[(1R,5S)-8-AZABICYCLO[3.2.1]OCTAN-3-YL] BENZOATE | C14 H17 N O2 | 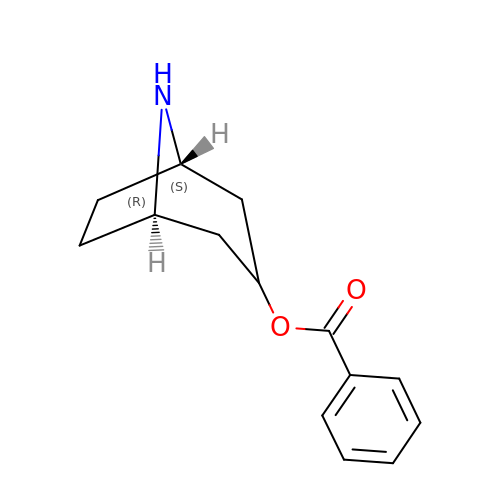AZHSHGVBEAPALY-ITGUQSILSA-N Rspo (R-spondin, also roof plate-specific spondin) proteins are evolutionarily conserved from fish to humans and have well-documented roles in a broad range of developmental and physiological processes resulting from enhancement of canonical and non-canonical Wnt signalling. ZNRF3/RNF43 specifically targets these Wnt receptors for ubiquitination and turnover, hence reducing Wnt signalling responses. Direct extracellular interaction with Rspo proteins inhibits ZNRF3/RNF43 activity. Here we report a molecular level analysis of the ZNRF3/RNF43 ectodomain structure and its interactions with Rspo proteins.

The ZNRF3ecto crystal structures revealed a distinctive variant of the protease-associated domain topology. All but two of these crystal structures reveal an extensive interface (average interface area 992±109 Å2) formed between two ZNRF3ecto polypeptide chains. The interaction is twofold symmetric; strands β3 and β7 of the ‘subunits’ abut face-to-face at the core of the dimer. Formation of the observed crystallographic ZNRF3 dimer in solution is further supported by the observation of almost quantitative spontaneous crosslinking of the S90C variant of mZNRF3ecto that introduces a cysteine close to the dimer symmetry axis. A crystal structure of this variant at 2.1 Å shows that this mutation and crosslinking is easily accommodated, requiring only minor backbone distortions. Ligand binding leads to a structuring of the acidic region of the β3–β4 loop. This same region of the β3–β4 loop also interacts with the β1–β2 hairpin in the opposing subunit of the ZNRF3ecto dimer. Notably, the β1–β2 hairpin shows less conformational variation in the liganded ZNRF3ecto dimer structures, always maintaining a tight embrace, consistent with the Rspo2Fu1–Fu2 interactions contributing an indirect stabilizing effect on the dimer via the β3–β4 loop. This stabilizing effect provides an explanation for our results showing that Rspo2Fu1–Fu2 bound weaker to monomerized mZNRF3ecto E92N, E94T but stronger to predimerized mZNRF3ecto S90C than to the wt mZNRF3ecto. Consistent with these co-immunoprecipitation data, Rspo2Fu1–Fu2 simultaneously bound to ZNRF3 and LGR5 in SPR binding assays with the monomerized ZNRF3ecto binding weaker and the dimerized S90C variant binding stronger to a preformed LGR5ecto–RspoFu1–Fu2 complex.

> ETGKETAFVEVVLFESSPSGDYTTHTTGLTGRFSRAGAMLCAEGEIVQMHPLGLCNNNDEEDLYEYGWVGVVKLEQPELDPKPCLTVLGKAKRAVQRGATAVIFDVSENPEAIDQLNQGSEDPLKRPVVYVKGADAIKLMNIVNKQKVARARIQHLGTKHHHHHH> QDISLSCGASEPAVDQDKKKWEPDTKFLKTPNTVHAPATYQDPSLLSTVPYMTSRIFTAPATYEIPVKGDKRHMLRLHFYPSTYTGLNILDSYFSVAANDLTLLSNFSAAITCQALTQAYLVREYSLAPSEKDVLSIIFTPSDKHPKAFAFINGIEVIPMPELFDTASLVGFSDQTSDTKTANLQTMFRLNVGGQDIPGSQDSGGLTRTWYNDAPYIFSAGLGVTLQASNNFRIDYQKMPVSTAPADVYKTARSQGPNGDINMKSNLTWMFQVDTNFTYIMRLHFCEFQLAKINQKVFNIFINNRTAQGDTNPADILGWTGGKGIPTYKDYAIYVDANTGGGGEEISLQMTPSTFGQPEYYDSQ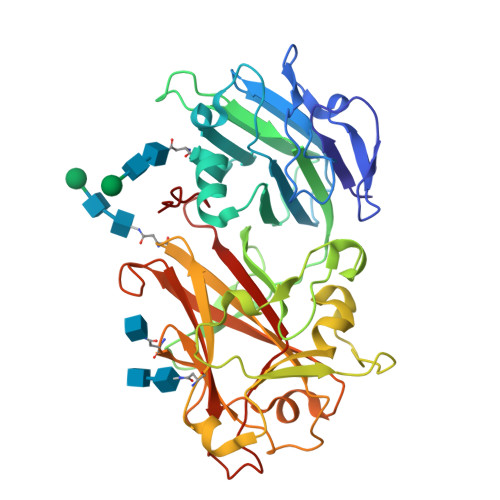LNGLEIFKIDTMKNLAGPNPKPS>MNPNQKIITIGSVSLIIATVCFLMQIAILVTTVTLHFKQHECDSPSSNQVMLCEPIIIERNITEIVYLNNTTIEKETCPKLVEYRNWSKPQCKITGFAPFSKDNSIRLSAGGDIWVTREPYVSCDPGKCYQFALGQGTTLDNKHSNDTIHDRIPHRTLLMNELGVPFHLGTRQVCIAWSSSSCHDGKAWLHVCVTGDDKNATASFIYDGRLVDSIGSWSQNILRTQESECVCINGTCTVVMTDGSASGRADTRILFIEEGKIVHISPLSGSAQHVEECSCYPRYPDVRCICRDNWKGSNRPIVDINMKDYSIDSSYVCSGLVGDTPRNDDRSSKSNCRNPNNERGNHGVKGWAFDNGNDVWMGRTISKDLRSGYETFKVIGGWSTPNSKSQINRQVIVDSDNRSGYSGIFSVEGKSCINRCFYVELIRGREQETRVWWTSNSIVVFC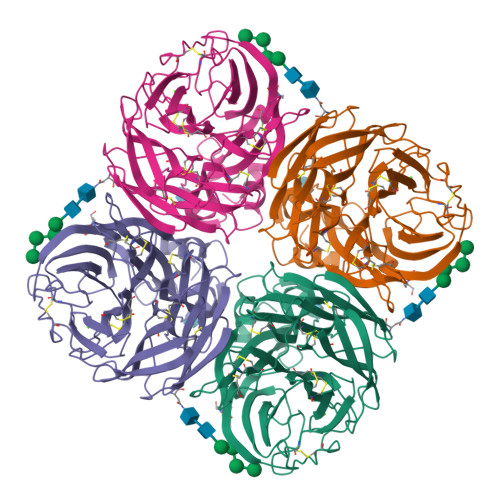GTSGTYGTGSWPDGANINFMPI[4x]N-[4-({[(6S)-2,4-diamino-5,6,7,8-tetrahydropyrido[3,2-d]pyrimidin-6-yl]methyl}amino)benzene-1-carbonyl]-L-glutamic acid | C20 H25 N7 O5 | 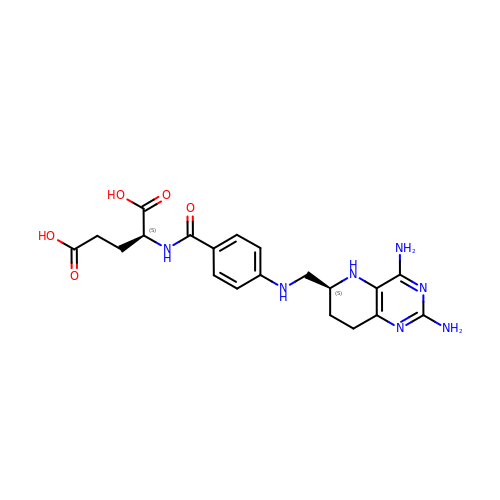NJZPEYYRVZHUEO-JSGCOSHPSA-N>[2x]GMVRISIAGGNEIDPGSMGLTLFHEHLRLITEVVRWNWP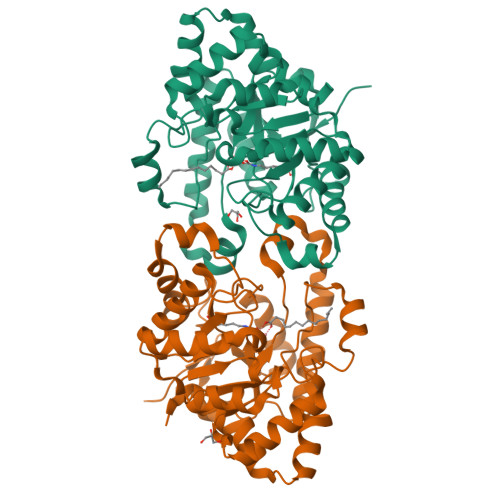HLYNEDEELKRAIDAVNAAKKYGVKTIIDLTVAGIGCDVRFNEKVAKATGVNIIMGTGFYTYTEIPFYFKNRGIDSLVDAFVHDITIGIQGTNTRAAFVKAVIDSSGLTKDVEMAIRAAAKAHIKTDVPIITHSFVGNKSSLDLIRIFKEEGVDLARTVIGHVGDTDDISFIEQILREGAFIGLDRFGLDIYLPLDKRVKTAIELIKRGWIDQLLLSHDYCPTIDWYPPEVVRSTVPDWTMTLIFEKVIPRMRSEGITEEQINRVLIDNPRRLFTGR[(2R)-5-(3-fluorophenyl)-2-{2-[hydroxy(methyl)amino]-2-oxoethyl}pentyl]phosphonic 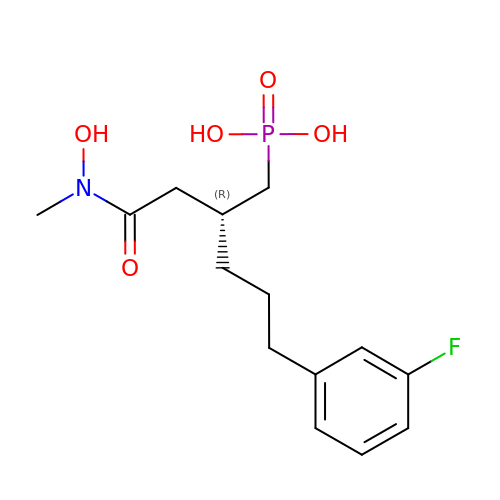acid | C14 H21 F N O5 P | HGIGLZBKPPPKTL-GFCCVEGCSA-N> EVKPKNKARRRTTTQMELL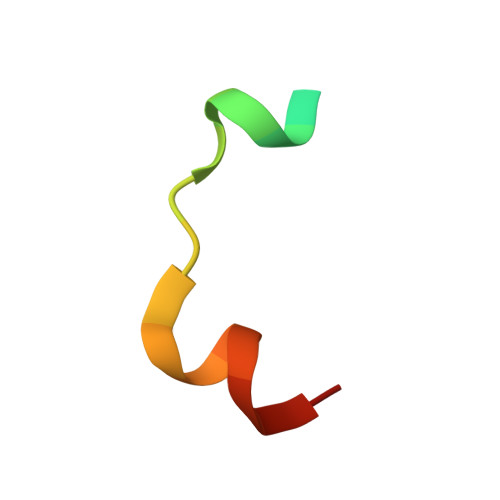YAD> MDYKDDDDKLEVLFQGPGSMMCLECASAAAGGAEEEEADAERRRRRRGAQRGAGGSGCCGARGAGGAGVSAAGDEVQTLSGSVRRAPTGPPGTPGTPGCAATAKGPGAQQPKPASLGRGRGAAAAILSLGNVLNYLDRYTVAGVLLDIQQHFGVKDRGAGLLQSVFICSFMVAAPIFGYLGDRFNRKVILSCGIFFWSAVTFSSSFIPQQYFWLLVLSRGLVGIGEASYSTIAPTIIGDLFGIDCSFWNESYLTGSRDERKKSLLSKFGMDEGVTFMFIGRFDRGQKGVDVLLKAIEILSSKKEFQEMRFIIIGKGDPELEGWARSLEEKHGNVKVITEMLSREFVRELYGSVDFVIIPSYFEPFGLVALEAMCLGAIPIASAVGGLRDIITNETGILVKAGDPGELANAILKALELSRSDLSKFRENCKKRAMSFSTKNTRTLMLSVFYFAIPLGSGLGYITGSSVKQAAGDWHWALRVSPVLGMITGTLILILVPATKRGHADQLGDQLKARTSWLRDMKALIRNRSYVFSSLATSAVSFATGALGMWIPLYLHRAQVVQKTAETCNSPPCGAKDSLIFGAITCFTGFLGVVTGAGATRWC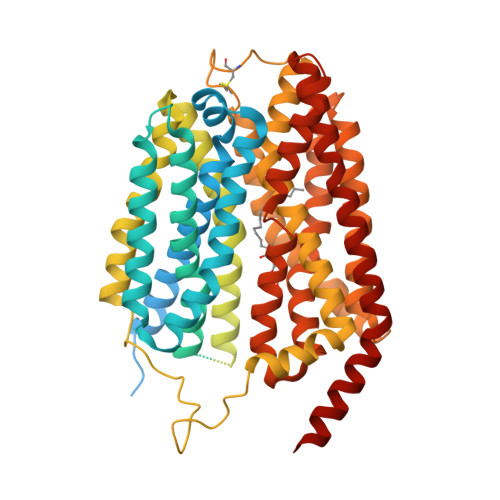RLKTQRADPLVCAVGMLGSAIFICLIFVAAKSSIVGAYICIFVGETLLFSNWAITADILMYVVIPTRRATAVALQSFTSHLLGDAGSPYLIGFISDLIRQSTKDSPLWEFLSLGYALMLCPFVVVLGGMFFLATALFFVSDRARAEQQVNQLAMPPASVKV Dodecin from Halobacterium salinarum is a hollow spherical dodecameric protein, which binds oxidized flavins with high affinity, whereas flavin reduction induces the dissociation of the holoprotein. Herein we use the riboflavin binding protein dodecin as a redox-sensitive probe to study ET processes through DNA monolayers. To study ET, dodecin can be reconstituted on flavin-terminated ds-DNA adsorbed on gold electrodes. If ET through DNA is possible, applying a negative potential will result in flavin reduction and subsequent release of apododecin.

Prior to adsorption of apododecin tE, a non-binding dodecin variant dA was added as a negative control to show that apododecin tE is bound specifically to the flavins.5b To minimize the ET distance between the redox-active isoalloxazine subunit of flavin and DNA, different flavin–DNA ligands comprising only the first five bases at the 5′ end (oligo 5, O5) and flavins of different lengths (CofCn) were synthesized. Dodecin was reconstituted with these ligands and X-ray structures were measured. In Figure 1 A the structures of the flavin–DNA ligands CofCn O5 with a hexyl, butyl, propyl, and ethyl group (n=6, 4, 3, 2) at the N(10) of the isoalloxazine moiety are shown. For all the flavin–DNA ligands, electron density can be traced for the isoalloxazine moiety (and the first two CH2 groups). For the CofC2_O5 ligand further electron density indicates binding between apoprotein and linker plus the first two DNA bases. As shown by superposition of the ligands in Figure 1 B, the (rather deep) position of the isoalloxazine ring of CofC2_O5 in the binding pocket is similar to that of lumiflavin, while all the other flavin–DNA hybrid ligands superimpose with riboflavin. For electrochemical measurements a ligand with n=3, bound only by its (oxidized) isoalloxazine moiety, appeared to be the best compromise between high affinity binding and short ET distance. Efficient ET could be observed even for larger distances between isoalloxazine and “molecular wires”, when the flavoenzyme glucose oxidase was reconstituted on gold electrodes, but using molecules other than DNA (e.g. single-walled carbon nanotubes) as the molecular wire.5f, 9 In the X-ray structures there was no electron density for most of the linker between DNA and flavin indicating that (also after protein reconstitution) different orientations of DNA and redox-center relative to each other are possible.

> MVFKKVLLTGTSEESFTAAADDAIDRAEDTLDNVVWAEVVDQGVAIGAVRTYQTEVQVAFELDGSQLEHHHHHH>GAMAPPRKVLIISAGASHSVALLSGDIVCSWGRGEDGQLGHGDAEDRPSPTQLSALDGHQIVSVTCGADHTVAYSQSGMEVYSWGWGDFGRLSHGNSSDLFTPLPIKALHGIRIKQIACGDSHCLAVTMEGEVQSWGRNQNGQLGLGDTEDSLVPQKIQAFEGIRIKMVAAGAEHTAAVTEDGDLYGWGWGRYGNLGLGDRTDRLVPERVTSTGGEKMSMVACGWRHTISVSYSGALYTYGWSKYGQLGHGDLEDHLIPHKLEALSNSFISQISGGARHTMALTSDGKLYGWGWNKFGQVGVGNNLDQCSPVQVRFPDDQKVVQVSCGWRHTLAVTERNNVFAWGRGTNGQLGIGESVDRNFPKIIEALSVDG[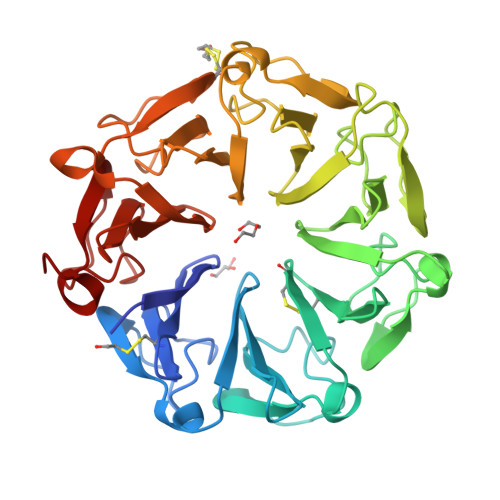2x]> MAVSKRPFSINSFAVNLNIGNFVDARYWSKCSKIEKTYNTGEYSDGQSNIIYTLPGAIKYPEVVLSKAFSPGDEELINRLIAV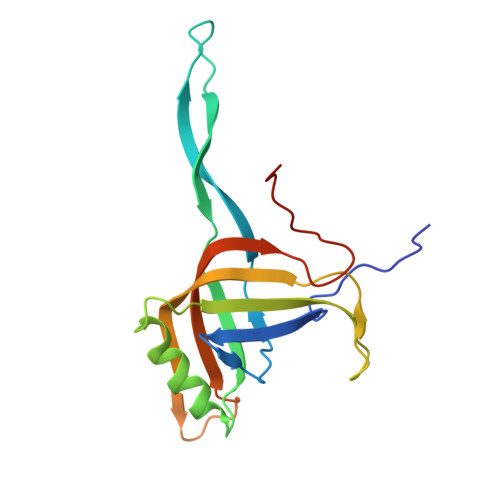NSDPIAWVTVFIQPMYRDGYYNVPQGGKIILEFCTVARATPINEIDTIGSNAAMFECALNPSRIRSDGGNINWWSEPAAQVAEF> ADVCMDPEPIVRIVGRNGLCVDVTGEEFFDGNPIQLWPCKSNTDWNQLWTLRKDSTIRSNGKCLTISKSSPRQQVVIYNCSTATVGATRWQIWDNRTIINPRSGLVLAATSGNSGTKLTVQ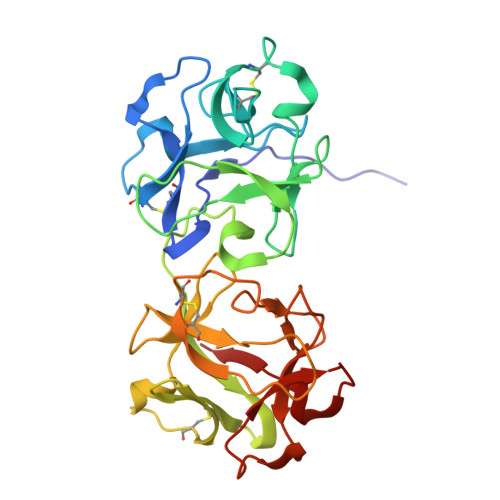TNIYAVSQGWLPTNNTQPFVTTIVGLYGMCLQANSGKVWLEDCTSEKAEQQWALYADGSIRPQQNRDNCLTTDANIKGTVVKILSCGPASSGQRWMFKNDGTILNLYNGLVLDVRRSDPSLKQIIVHPFHGNLNQIWLPLF> SGLQGHIIENPQYFSDACVHHIKRRDIVLKWELG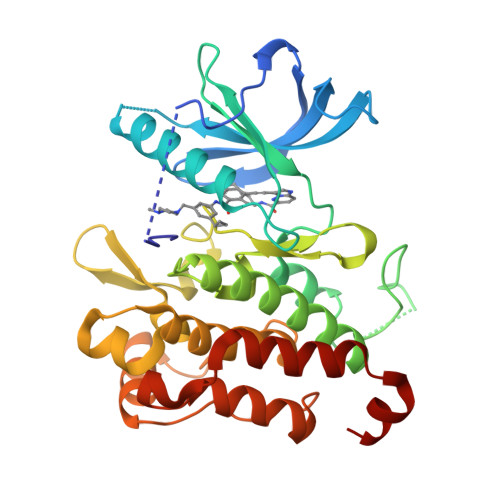EGAFGKVFLAECHNLLPEQDKMLVAVKALKEASESARQDFQREAELLTMLQHQHIVRFFGVCTEGRPLLMVLEYMRHGDLNRFLRSHGPDAKLLAGGEDVAPGPLGLGQLLAVASQVAAGMVYLAGLHFVHRDLATRNCLVGQGLVVKIGDFGMSRDIYSTDYYRVGGRTMLPIRWMPPESILYRKFTTESDVWSFGVVLWEIFTYGKQPWYQLSNTEAIDCITQGRELERPRACPPEVYAIMRGCWQREPQQRHSIKDVHARLQALAQAPPVYLDVLG>MAIFGELSSLGHLFKKTQELEILHEYLKEVMQKGSKANQRVLNLATNTEFQVPLGHGIFSIEQSYCLEHAKESEKGFFESHKKYVDFQLIVKGVEGAKAVGINQAVIKNPYDEKRDLIVYEPVSEASFLRLHAGMLAIFFENDAHALRFYGESFEKYREEPIFKAVVKAPKGLIKLKLAAENLYF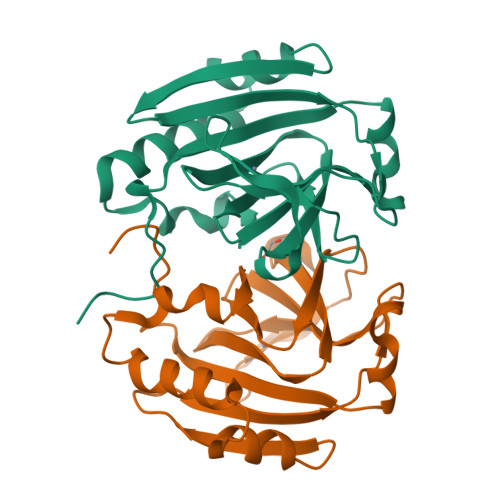QGIDHHHHHH[2x]C-reactive protein (CRP) is a pentameric protein of 115 kDa composed of five identical non-covalently associated pentraxin domains. The B-face binds to a range of ligands, with the canonical example being phosphocholine (PCh) head groups in lipids such as phosphatidylcholine. This is a calcium-dependent interaction, with each CRP monomer chelating two adjacent Ca2+ ions. The A-face modulates many effector functions of CRP, such as activation of the classical complement pathway, where binding of complement component C1q to CRP is mediated via predominantly electrostatic interactions between the Ca2+-containing globular head domain of C1q (gC1q) and the A-face of CRP.

Decameric CRP is formed from the offset stacking of two pentamers via their A-faces. Intermolecular contacts between monomers within CRP decamers were also dominated by non-covalent ionic bonds, which formed a second ionic zipper, perpendicular to that found in CRP pentamers. Ionic bonds included Asp163(chain A)–Arg188(J), Glu170(A)–Arg6(J), Arg188(E)–Asp163(F), Arg188(B)–Asp169(H) and Asn172(C)–Ser181(G). Although decamers appeared to adopt C2 symmetry, they were solved without symmetry applied and reached resolutions of 3.3 – 2.8 Å. In all maps of pentameric and decameric CRP, clear density was present for two Ca2+ ions, and in conditions including PCh density for the ligand was visible and adopted similar conformations between the cryoEM derived models and those found in crystal structures. In contrast, there was a slight increase in the prevalence of pentamers at pH 7.5 when in the presence of PCh. The addition of PCh amplified this difference, with pH 5 containing 93.3% decamers vs 40% at pH 7.5. No major differences were observed between the decamers at different pHs, with or without PCh, other than the proportions of decamers to pentamers.

>[10x]QTDMSRKAFVFPKESDTSYVSLKAPLTKPLKAFTVCLHFYTELSSTRGYSIFSYATKRQDNEILIFWSKDIGYSFTVGGSEILFEVPEVTVAPVHICTSWESASGIVEFWVDGKPRVRKSLKKGYTVGAEASIILGQEQDSFGGNFEGSQSLVGDIGNVNMWDFVLSPDEINTIYLGGPFSPNVLNWRALKYEVQGEVFTKPQLWP>[2x]MAHLLHIDSSISGPASVSRPLTARAAANWKAAHPDGTVTYRDLGASPLPHINTASALAGVTPAAERRPEQSAAWAVSELVVEEVREATTIILGLPLYNYG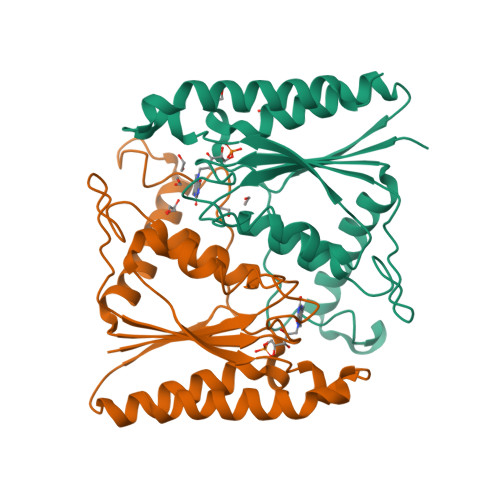PPSSVKAWVDYLIAPGLSLDAHTRAPLLGRRELLVLATRGGGFGPGTPREGWDHAQPWLPHGLAMTGLEPEFITTELTLAPVTPGMEHLVPLAKESRAAAERAIDQRWVTSLVR(4R)-2'-amino-6-bromo-1',2,2-trimethyl-2,3-dihydrospiro[chromene-4,4'-imidazol]-5'(1'H)-one | C14 H16 Br N3 O2 | 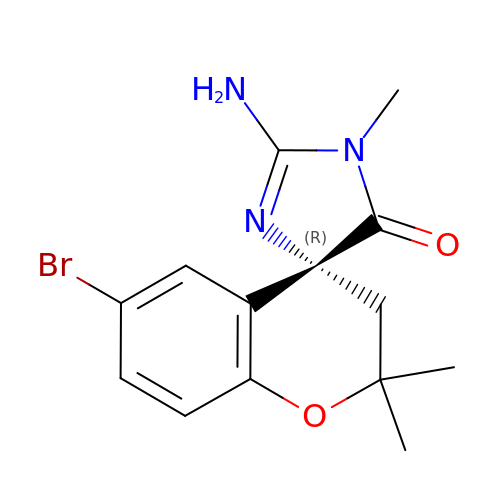GCJNGEZDKLVQNN-CQSZACIVSA-N> MTNPSNSNLQALREELCTPGLDQGHLFEGWPETVDECNERQIALLTDLYMFSNMYPGGVAQYIRNGHELLARESEEVDFAALEMPPLIFEAPSLHRRTAERTALENAGTAMLCKTVFVLVAGGLGERLG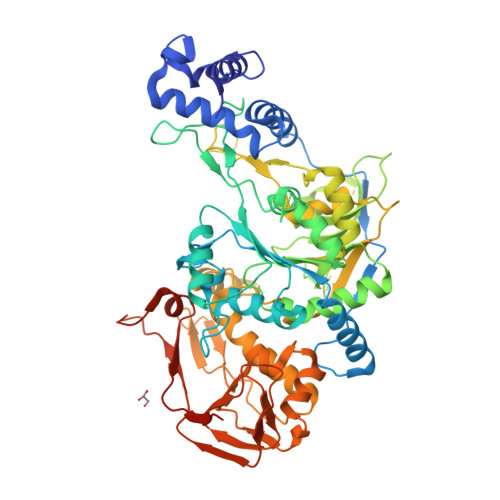YSSIKVSLPVETATNTTYLAYYLRWAQRVGGKEVPFVIMTSDDTHDRTLQLLRELQLEVPNLHVLKQGQVFCFADSAAHLALDETGKLLRKPHGHGDVHSLIYNATVKRDVVPDSGDGTATAQPLVNDWLAAGYESIVFIQDTNAGATITIPISLALSAEHSLDMNFTCIPRVPKEPIGLLCRTKKNSGDPWLVANVEYNVFAEVSRALNKDGGDEVSDPTGFSPFPGSVNTLVFKLSSYVDRLRESHGIVPEFINPKYSDETRRSFKKPARIESLMQDIALLFSEDDYRVGGTVFERFSYQPVKNSLEEAAGLVAQGNGAYCAATGEAAFYELQRRRLKAIGLPLFYSSQPEVTVAKDAFGVRLFPIIVLDTVCASSGSLDDLARVFPTPEKVHIDQHSTLIVEGRVIIESLELYGALTIRGPTDSMALPHVVRNAVVRNAGWSVHAILSLCAGRDSRLSEVDRIRGFVLKKTAMAVMDCNTKGESEAGAPSGAADPAKL> MKLKTIAVACSALMMLSGASAVMAYDGTKCKAAGDCWEAKPGFPDKIKG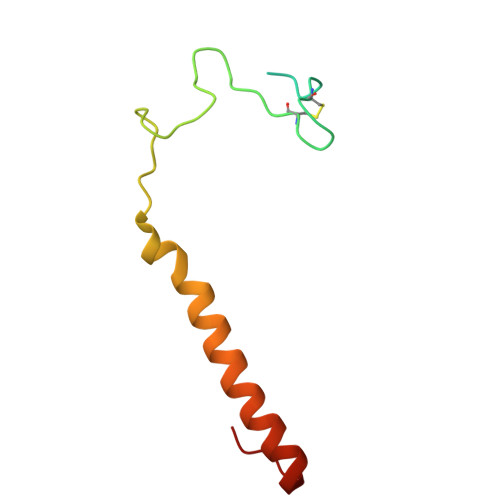SKYDPKHSEKELNKQDAALKAMEKRNAERVEQFKKTGKWVY>[2x]MSSFVPNKEQTRTVLIFCFHLKKTAAESHRMLVEAFGEQVPTVKTCERWFQRFKSGDFDVDDKEHGKPPKRYEDAELQALLDEDDAQTQKQLAEQLEVSQQAVSNRLREMGKIQKVGRWVPHELNERQMERRKNTCEILLSRYKRKSFLHRIVTGDEKWIFFVNPKRKKSYVDPGQPATSTARP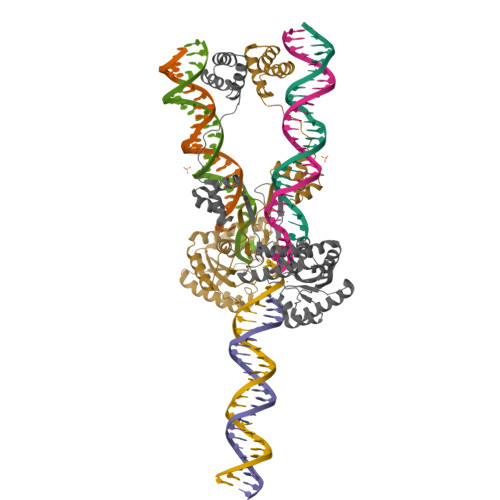NRFGKKTMLCVWWDQSGVIYYELLKPGETVNAARYQQQLINLNRALQRKRPEYQKRQHRVIFLHDNAPSHTARAVRDTLETLNWEVLPHAAYSPDLAPSDYHLFASMGHALAEQRFDSYESVKKWLDEWFAAKDDEFYWRGIHKLPERWEKCVASDGKYFE>[2x]MTIDEIIEAIEKLTVSELAELVKKLEDKFGVTAAAPVAVAAAPVAGAAAGAAQEEKT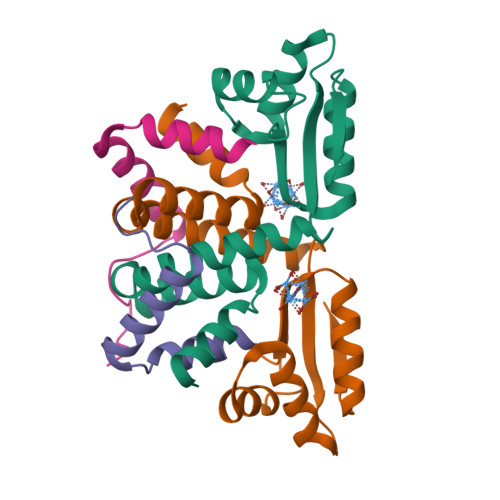EFDVVLKSFGQNKIQVIKVVREITGLGLKEAKDLVEKAGSPDAVIKSGVSKEEAEEIKKKLEEAGAEVELK;>MTIDEIIEAIEKLTVSELAELVKKLEDKFGVTAAAPVAVA[2x]5-[[6-chloranyl-3-[3-(4-chloranyl-3,5-dimethyl-phenoxy)propyl]-7-(3,5-dimethyl-1~{H}-pyrazol-4-yl)-1~{H}-indol-2-yl]carbonylsulfamoyl]furan-2-carboxylic 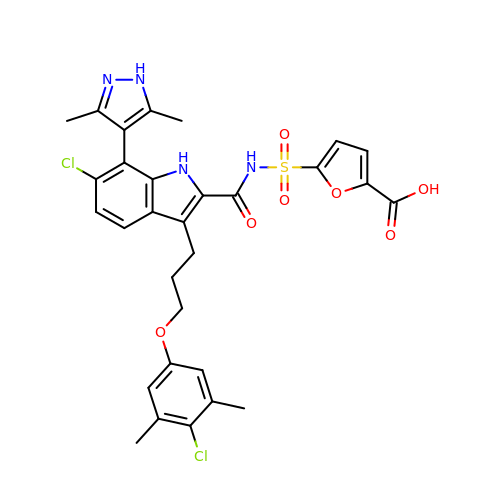acid | C30 H28 Cl2 N4 O7 S | KTNNYAXNCQVPIU-UHFFFAOYSA-N> 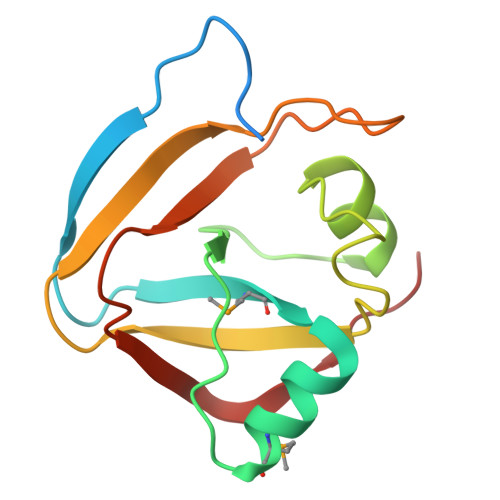MGSSHHHHHHSQDPNSAWLEGTQVKTEIVPPGRQYQMVVAKGQAEAIMQGKPAFGGFAAPEPIPSQAYARDKLVILDRFKTDVSHVITVETTAPQKIHSGITGPLENYKGGVQQVEFVGDRNLKIVGTPGVLPVE> TRVVYKVPEEQPPNTLIGSLAADYGFPDVGHLYKLEVGAPYLRVDGKTGDIFTTETSIDREGLRECQNQLPGDPCILEFEVSITDLVQNGSPRLLEGQIEVQDINDNTPNFASPVITLAIPENTNIGSLFPIPLASDRDAGPNGVASYELQAGPEAQELFGLQVAEDQEEKQPQLIVMGNLDRERWDSYDLTIKVQDGGSPPRASSALLRVTVLDTNDNAPKFERPSYEAELSENSPIGHSVIQVKANDSDQGANAEIEYTFHQAPEVVRRLLRLDRNTGLITVQGPVDREDLSTLRFSVLAKDRGTNPKSARAQVVVTVKDMNDNAPTIEIRGIGLVTHQDGMANISEDVAEETAVALVQVSDRDEGENAAVTCVVAGDVPFQLRQASETGSDSKKKYFLQTTTPLDYEKVKDYTIEIVAVDSGNPPLSSTNSLKVQVVDVNDNATDPPVGGHHHHHH

Protocadherin-1 (PCDH1) is a non-clustered δ1 protocadherin involved in respiratory diseases. PCDH1 has seven EC repeats (labeled EC1 to EC7 from N to C-terminus), a single pass transmembrane domain and a cytoplasmic domain with the three conserved motifs (CM1–CM3) typical of the δ1 subgroup. PCDH1 may bind bronchial epithelial cells and epithelial cells of the airway mucosa together by mediating homophilic adhesion and helping in forming the epithelial barrier. Here we use bead aggregation assays to show that repeats EC1 to EC4 form the minimal adhesive unit for human (Homo sapiens [hs]) PCDH1, despite its longer extracellular domain with seven EC repeats.

The third one, PCDH1 EC1-4mc at 3.15 Å, was obtained using protein produced by mammalian cells. The PCDH1 EC1-4mc structure had regions in which electron density could only be explained by the presence of glycosylation. Residues N89, N248, and N346 are predicted to be N-linked glycosylation sites and sugars can be observed at N248 in the PCDH1 EC1-4mc structure. C-linked glycosylation has been predicted for W186 but is not observed in our structure, while O-linked glycosylation has not been predicted but it is observed at S430. The observed O-linked glycosylated residue S430 is also near the PCDH1-I2 interface. However, sugars observed at N248 and S430 did not interfere with this interface in the crystal. We could not detect structural differences caused by glycosylation, and thus the role of these glycosylation sites in PCDH1 function remains unclear. An additional calcium ion near the EC2–EC3 linker is unique, it is at a crystal contact, and it might be present due to purification and crystallization conditions with high calcium. The PCDH1 EC1-4mc structure does not have this additional calcium ion.>RSSNELHQVPSNCDCLNGGTCVSNKYFSNIHWCNCPKKFGGQHCEIDKSKTCYEGNGHFYRGKASTDTMGRPCLPWNSATVLQQTYHAHRSDALQLGLGKHNYCRNPDNRRRPWCYVQVGLKPLVQECMVH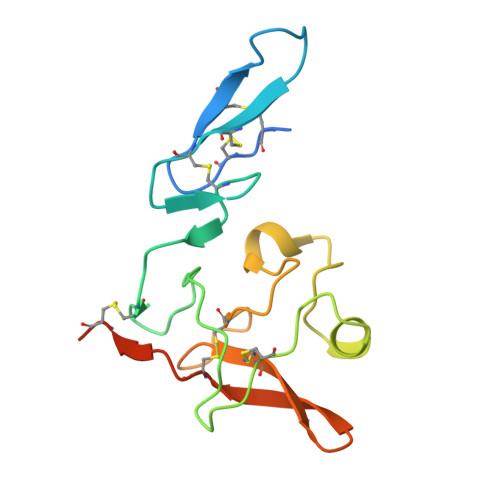DCADGKKPSSPPEE[4x]>[12x]TRDQNGTWEMES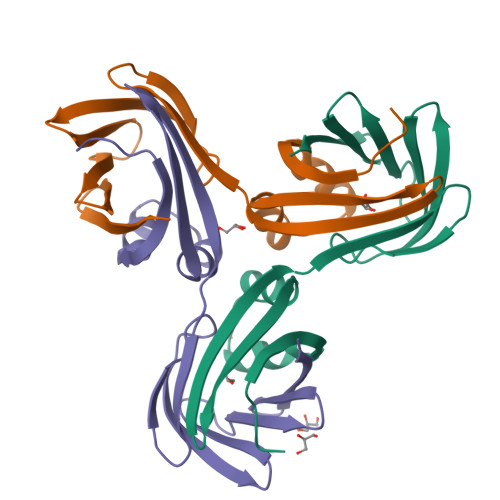NENFEGYMKALDIDFATRKIAVRLTQTKVIDQDGDNFKDKTTSTFRNYDVDFTVGVEFDEYTKSLDNRHVKALVTWEGDVLVCVQKGEKENRGWKKWIEGDKLYLELTCGDQVCRQVFKKK>[4x]GAMGSMAEAEGESLESWLNKATNPSNRQEDWEYIIG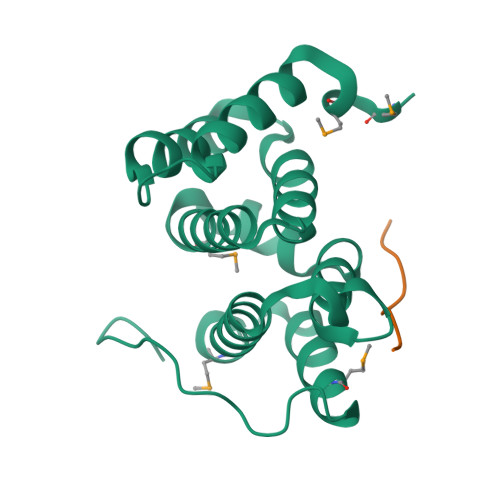FCDQINKELEGPQIAVRLLAHKIQSPQEWEALQALTVLEACMKNCGRRFHNEVGKFRFLNELIKVVSPKYLGDRVSEKVKTKVIELLYSWTMALPEEAKIKDAYHMLKRQGIVQSDPPIPVDRTLIPSPPPRPKN;>[4x]FHDDSDEDLLHI(1S)-2,2-difluoro-N-[(1S,5R,6R)-3-{5-fluoro-2-[(1-methyl-1H-pyrazol-4-yl)amino]pyrimidin-4-yl}-6-methyl-3-azabicyclo[3.1.0]hexan-1-yl]cyclopropane-1-carboxamide | C18 H20 F3 N7 O | 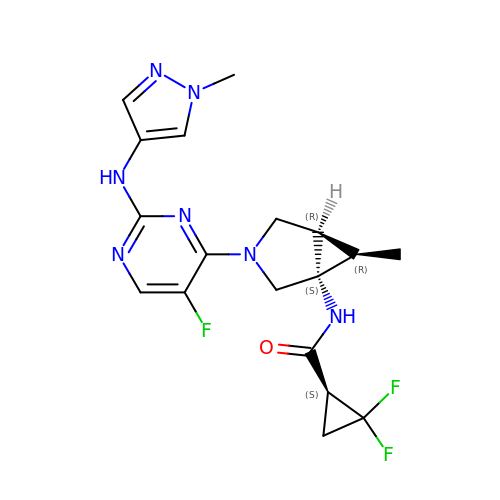VFTQZQGHFFDMQS-RSNHQYPWSA-N> AAATSLVYDTCYVTLTERATTSFQRQSFPTLKGMGDRAFQVVAFTIQGVSAAPLMYNARLYNPGDTDSVHATGVQLMGTVPRTVRLTPRVGQNNWFFGNTEEAETILAIDGLVSTKGANAPSNTVIVTGCFRLAPSEL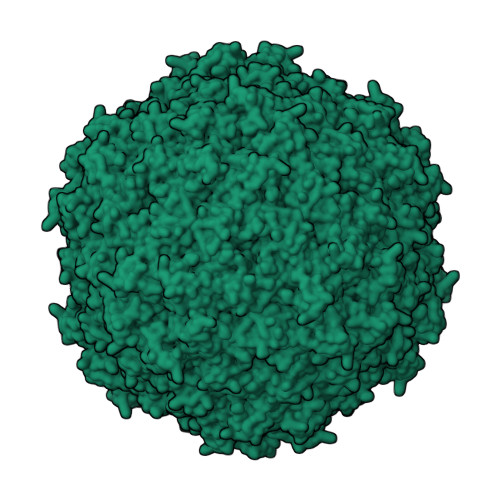QSS>[2x]GSHMLDRRSDKRNNSDWLQAKESHPTTVYLLFSDLNPLVTLGGNKESSQQPEVRLCQLNYPDVKGYLAQPEKITLVFLGVELEMRKGSPAQAGGVPEAAADGLVAWFALGIEPGAAEEFKQRHENCYFLHPPMPALLQLKEKEAGVVAQARSVLAWHSRYKFCPTCGSATKIEEGGYKRVCVRETCPSLQGV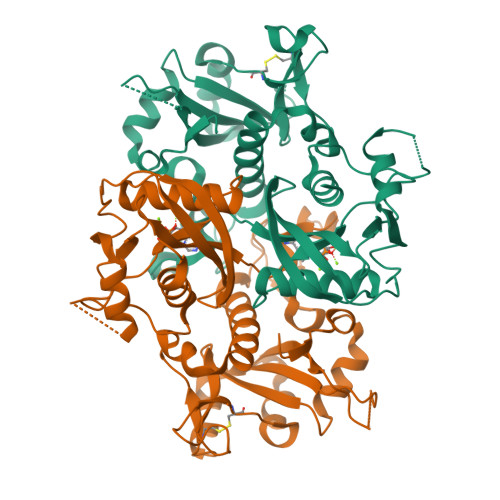HNTSYPRVDPVVIMQVIHPDGTKCLLGRQKRFPPGMFTCLAGFIEPGETIEDAVRREVEEESGVKVGHVQYVSCQPWPMPSSLMIGCLAVAVSTEIKVDKNEIEDARWFTREQVVDVLTKGKQQAFFVPPSRAIAHQLIKHWVGMNP>SNAMFCYQCQETVGNKGCTQVGVCGKKPETAALQDALIYVTKGLGQIATRLRAEGKAVDHRIDRLVTGNLFATITNANFDDDILAERVRMTCAAKKELAASLTDKSGLSDAALWEASEKSAMLAKAGTVGVMATTDDDVRSL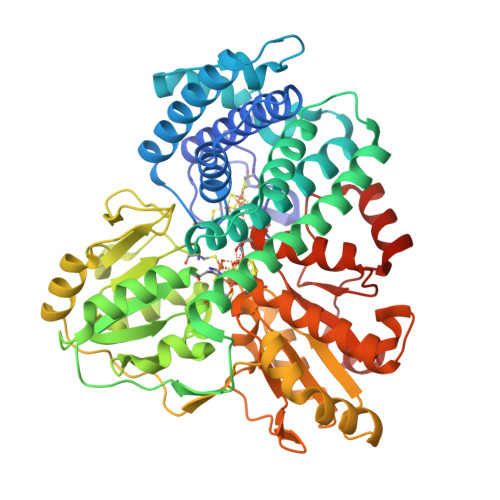RWLITFGLKGMAAYAKHADVLGKHENSLDAFMQEALAKTLDDSLSVADLVALTLETGKFGVSAMALLDAANTGTYGHPEITKVNIGVGSNPGILISGHDLRDLEMLLKQTEGTGVDVYTHSEMLPAHYYPAFKKYAHFKGNYGNAWWKQKEEFESFNGPVLLTTNCLVPPKDSYKDRVYTTGIVGFTGCKHIPGEIGEHKDFSAIIAHAKTCPAPTEIESGEIIGGFAHNQVLALADKVIDAVKSGAIKKFVVMAGCDGRAKSRSYYTDFAEGLPKDTVILTAGCAKYRYNKLNLGDIGGIPRVLDAGQCNDSYSLAVIALKLKEVFGLEDVNDLPIVYNIAWYEQKAVIVLLALLSLGVKNIHLGPTLPAFLSPNVAKVLVEQFNIGGITSPQDDLKAFFG[2x]> MSLSNKLTLDKLDVKGKRVVMRVDFNVPMKNNQITNNQRIKAAVPSIKFCLDNGAKSVVLMSHLGRPDGVPMPDKYSLEPVAVELKSLLGKDVLFLKDCVGPEVEKACANPAAGSVILLENLRFHVEEEGKGKDASGNKVKAEPAKIEAFRASLSKLGDVYVNDAFGTAHRAHSSMVGVNLPQKAGGFLMKKELNYFAKALESPERPFLAILGGAKVADKIQLINNMLDKVNEMIIGGGMAFTFLKVLNNMEIGTSLFDEEGAKIVKDLMSKAEKNGVKITLPVDFVTAD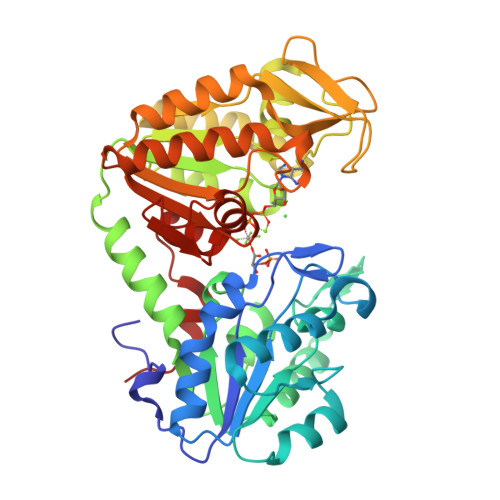KFDENAKTGQATVASGIPAGWMGLDCGPESSKKYAEAVTRAKQIVWNGPVGVFEWEAFARGTKALMDEVVKATSRGCITIIGGGDTATCCAKWNTEDKVSHVSTGGGASLELLEGKVLPGVDALSNI> MTIKTKAELLNKWKPLLEGEGLPEIANSKQAIIAKIFENQEKDFQTAPEYKDEKIAQAFGSFLTEAEIGGDHGYNATNIAAGQTSGAVTQIGPAVMGMVRRAIPNLIAFDICGVQPMNSPTGQVFALRAVYGKDPVAAGAKEAFHPMYGPDAMFSGQGAAKKFPALAASTQTTVGDIYTHFFQETGTVYLQASVQVTIDAGATDAAKLDAEIKKQMEAGALVEIAEGMATSIAELQEGFNGSTDNPWNEMGFRIDKQVIEAKSRQLKAAYSIELAQDLRAVHGMDADA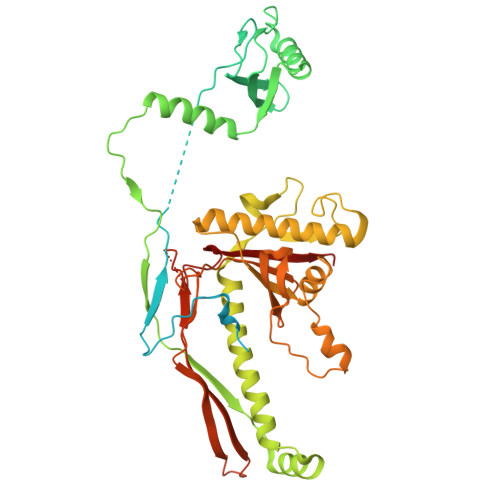ELSGILATEIMLEINREVVDWINYSAQVGKSGMTLTPGSKAGVFDFQDPIDIRGARWAGESFKALLFQIDKEAVEIARQTGRGEGNFIIASRNVVNVLASVDTGISYAAQGLATGFSTDTTKSVFAGVLGGKYRVYIDQYAKQDYFTVGYKGPNEMDAGIYYAPYVALTPLRGSDPKNFQPVMGFKTRYGIGINPFAESAAQAPASRIQSGMPSILNSLGKNAYFRRVYVKGI> MEAGITGTWYNQLGSTFIVTAGADGALTGTYACGRGNAECRYVLTGRYDSAP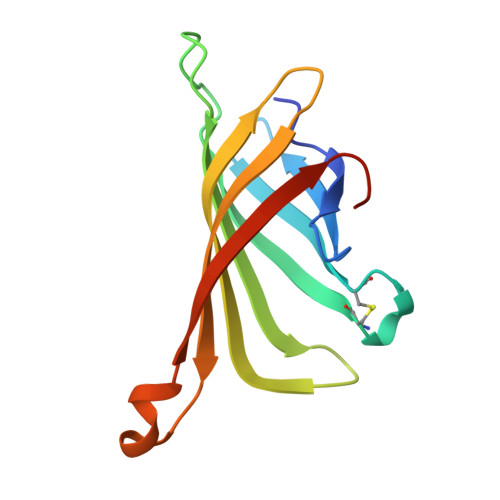ATDGSGTALGWTVAWKNNYRNAHSATTWSGQYVGGAEARINTQWLLTSGTTEANAWKSTLVGHDTFTKVKPSAAS> MRRFGSKFASGLASRCALACPLASAATAPAGASTTSSTSSAQKSFFKTTEMIGYVHSIDGTIATLIPAPGNPGVAYNTIIQIQVSPTTFAAGLVFNLEKDGRIGIILMDNITEVQSGQKVMATGQLLHIPVGAGVLGKVVNPLGHEVPVGLVTRSRRLLDSTLGKVDTGAPNIVSRSPVNYNLLTGFKAVDTMIPIGRGQRELIVGDRQTGKTSIAVSTIINQVRINQQILSKNAVISIYVSIGQRCSNVARIHRLLQSYGALRYTTVMAATAAEPAGLQYLAPYAGVTMGEYFMNRGRHCLCVYDDLSKQAVAYRQISLLLRRPPGREAYPGDVFYLHSRLLERAAMLSPGKGGGS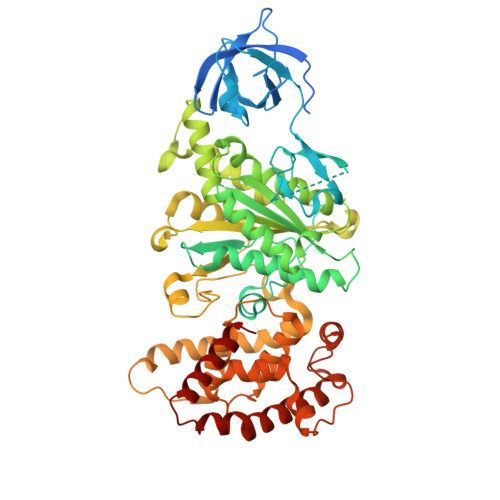VTALPIVETLSNDVTAYIVTNVISITDGQIYLDTKLFTGGQRPAVNIGLSVSRVGSSAQNAAMKGVAGKLKGILAEYRKLAADSVGGQQVQTIPMIRGARFVALFNQKQPSYFMNAIVSLYACLNGYLDDVKVQYVKFYEYLLVHRDLGIMYGTAKNKFFYMYVQELNYLIRFFTLNSPILHGELEEMLKQHTHLFLQHYQSKMNAIKSEKDVKALKNLLYSCKRAV Lysine crotonylation (Kcr) is a newly discovered histone PTM that is specifically enriched at active gene promoters and potential enhancers in mammalian cell genomes. We identified human Sirt1, Sirt2, and Sirt3 as decrotonylases in vitro and examined the molecular basis for how the enzymes recognize Kcr using X-ray crystallography. It should be noted that Sirt3 was found to localize predominantly to mitochondria and was mainly involved in metabolic regulations through controlling protein acetylation dynamics. We have demonstrated that endogenous Sirt3 functions as an ‘eraser’ to regulate histone crotonylation in cells.

The asymmetric unit consists of six molecules, each containing one Sirt3–H3K4Cr complex. The two globular domains of Sirt3 composed of an NAD binding Rossmann fold and a zinc binding motif are similar to other sirtuins. Residues 2RTKQTAR8 of the H3K4Cr peptide were clearly identified based on electron density. The crotonyl lysine is located in a binding pocket formed by hydrophobic residues Phe180, Ile230, His248, Ile291, and Phe294 of Sirt3. Residue His248, a catalytic residue for the deacetylation activity of Sirt3, interacts with the crotonyl amide oxygen via hydrogen bonding in the structure. Strikingly, the phenyl ring of residue Phe180 aligns parallel to the planar crotonyl group and has a short distance of 3.6 Å to its conjugated carbon–carbon double bond (C=C), indicating a robust π-π stacking interaction between the two functional groups. Interestingly, a primary sequence alignment of all sirtuins revealed that the phenylalanine residue (Phe180) of Sirt3 is conserved in Sirt1 and Sirt2, but not in other sirtuins, which may explain why Sirt4–Sirt7 were not identified in our CLASPI experiments. To further examine the importance of this conserved phenylalanine to the decrotonylase activity of the enzyme, we mutated Phe180 of Sirt3 to a leucine residue (F180L), which lacks an aromatic ring as a π donor but retains a similar hydrophobicity. The steady state kinetic data showed that the catalytic efficiency of Sirt3 F180L mutant (kcat/Km=21 s−1 M−1) for the hydrolysis of the H3K4Cr peptide was about 40-fold lower than that of wild-type Sirt3, indicating a critical role of the phenylalanine mediated π−π interaction in the decrotonylation activity of the enzyme. A mutation of the catalytic residue (H248Y) that is crucial for the deacetylation activity of the enzyme also completely abolished its decrotonylation activity. These data indicate that Sirt3 hydrolyzes crotonyl lysine with the same mechanism as it hydrolyzes acetyl lysine.

>[6x]GKLSLQDVAELIRARACQRVVVMVGAGISTPSGIPDFRSPGSGLYSNLQQYDLPYPEAIFELPFFFHNPKPFFTLAKELYPGNYKPNVTHYFLRLLHDKGLLLRLYTQNIDGLERVSGIPASKLVEAHGTFASATCTVCQRPFPGEDIRADVMADRVPRCPVCTGVVKPDIVFFGEPLPQRFLLHVVDFPMADLLLILGTSLEVEPFASLTEAVRSSVPRLLINRDLVGPLAWHPRSRDVAQLGDVVHGVESLVELLGWTEEMRDLVQRETGKLA;>RTKQTAR[6x]INOSINE-5'-DIPHOSPHATE | C10 H14 N4 O11 P2 | 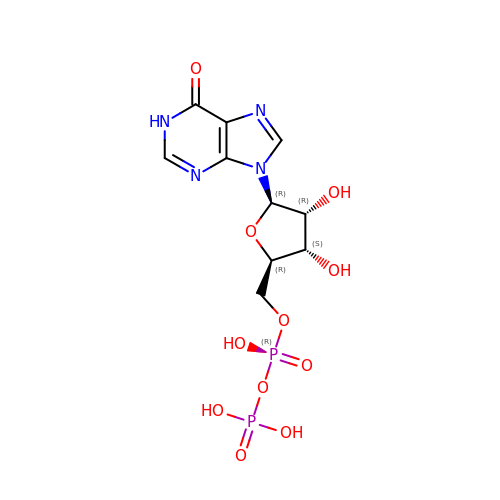JPXZQMKKFWMMGK-KQYNXXCUSA-N> GRSDAYTQVDNFLHAYARGGDELVNGHPSYTVDQAAEQILREQASWQKAPGDSVLTLSYSFLTKPNDFFNTPWKYVSDIYSLGKFSAFSAQQQAQAKLSLQSWSDVTNIHFVDAGQGDQGDLTFGNFSSSVGGAAFAFLPDVPDALKGQSWYLINSSYSANVNPANGNYGRQTLTHEIGHTLGLSHPGDYNAGEGDPTYADATYAEDTRAYSVMSYWEEQNTGQDFKGAYSSAPLLDDIAAIQKLYGANLTTRTGDTVYGFNSNTERDFYSATSSSSKLVFSVWDAGGNDTLDFSGFSQNQKINLNEKALSDVGGLKGNVSIAAGVTVENAIGGSGSDLLIGNDVANVLKGGAGNDILYGGLGADQLWGGAGADTFVYGDIAESSAAAPDTLRDFVSGQDKIDLSGLDAFVNGGLVLQYVDAFAGKAGQAILSYDAASKAGSLAIDFSGDAHADFAINLIGQATQ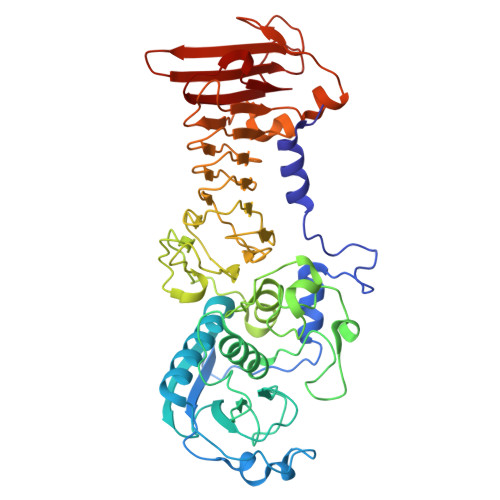ADIVV> REAVETAVRTLAEH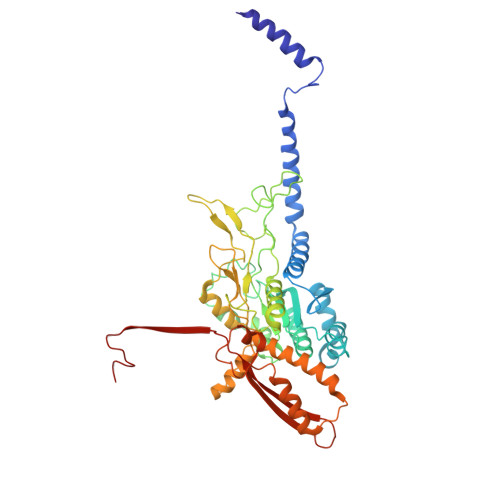ALEQTSLISNDAIKSIESIIAALDAKLTAQVNLIMHHADFQQLESAWRGLHYLVNNTETDEQLKIRVLNISKPELHKTLKKFKGTTWDQSPIFKKLYEEEYGQFGGEPYGCLVGDYYFDQSPPDVELLGEMAKISAAMHAPFISAASPTVMGMGSWQELSNPRDLTKIFTTPEYAGWRSLRESEDSRYIGLTMPRFLARLPYGAKTDPVEEFAFEEETDGADSSKYAWANSAYAMAVNINRSFKLYGWCSRIRGVESGGEVQGLPAHTFPTDDGGVDMKCPTEIAISDRREAELAKNGFMPLLHKKNTDFAAFIGAQSLQKPAEYDDPDATANANLAARLPYLFATCRFAHYLKCIVRDKIGSFKEKDEMQRWLQDWILNYVDGDPAHSTETTKAQHPLAAAEVVVEEVEGNPGYYNSKFFLRPHYQLEGLTVSLRLVSKLPSAKEA(5S)-3-(5,6-dihydro-2H-pyran-3-yl)-1-fluoro-7-(2-fluoropyridin-3-yl)spiro[chromeno[2,3-c]pyridine-5,4'-[1,3]oxazol]-2'-amine 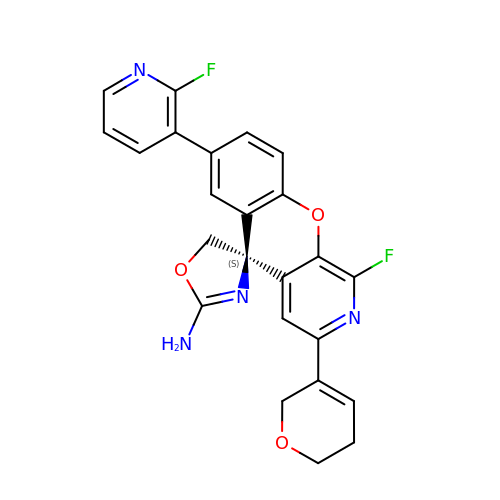| C24 H18 F2 N4 O3 | JAZOCUNZCUBRJX-DEOSSOPVSA-N(2R)-2-azanyl-4-methylsulfonyl-N-[3-(trifluoromethyloxy)phenyl]butanamide 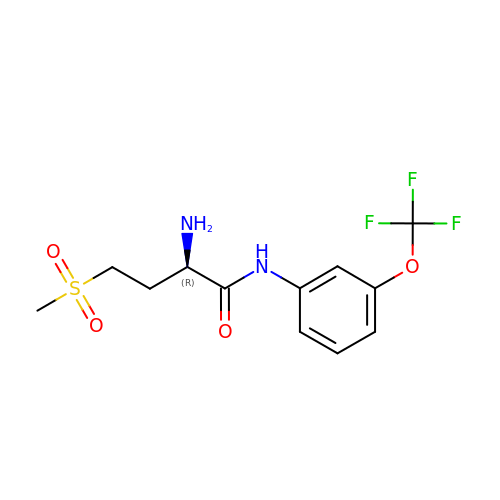| C12 H15 F3 N2 O4 S | SJCAGVRRCBPLMJ-SNVBAGLBSA-N> AAAASSST;> GLGQMLESMIDNTVRETVGAATSRDALPNTEASGPTHSKEIPALTAVETGATNPLVPSDTVQTRHVVQHRSRSESSIESFFARGACVTIMTVDNSASTTNKDKLFAVWKITYKDTVQLRRKLEFFTYSRFDMELTFVVTANFTETNNGHALNQVYQIMYVPPGAPVPEKWDDYTWQTSSNPSIFYTYGTAPARISVPYVGISNAYSHFYDGFSKVPLKDQSAALGDSLYGAASLNDFGILAVRVVNDHNPTKVTSKIRVYLKPKHIRVWCPRPPRAVAYYGP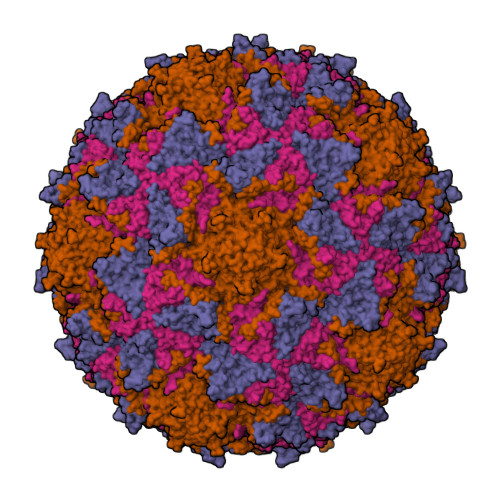GVDYKDGTLTPLSTKDLTTY;> SPNIEACGYSDRVLQLTLGNSTITTQEAANSVVAYGRWPEYLRDSEANPVDQPTEPDVAACRFYTLDTVSWTKESRGWWWKLPDALRDMGLFGQNMYYHYLGRSGYTVHVQCNASKFHQGALGVFAVPEMCLAGDSNTTTMHTSYQNANPGEKGGTFTGTFTPDNNQTSPARRFCPVDYLLGNGTLLGNAFVFPHQIINLRTNNCATLVLPYVNSLSIDSMVKHNNWGIAILPLAPLNFASESSPEIPITLTIAPMCCEFNGLRNITLPRLQ;> GLPVMNTPGSNQYLTADNFQSPCALPEFDVTPPIDIPGEVKNMMELAEIDTMIPFDLSATKKNTMEMYRVRLSDKPHTDDPILCLSLSPASDPRLSHTMLGEILNYYTHWAGSLKFTFLFCGSMMATGKLLVSYAPPGADPPKKRKEAMLGTHVIWDIGLQSSCTMVVPWISNTTYRQTIDDSFTEGGYISVFYQTRIVVPLSTPREMDILGFVSACNDFSVRLLRDTTHIEQKALAQ;> GAQVSSQKVGAHENSNRAYGGSTINYTTINYYRDSASNAASKQDFSQDPSKFTEPIKDVLIKTAPMLN> IIYPGTLWCGHGNKSSGPNELGRFKHT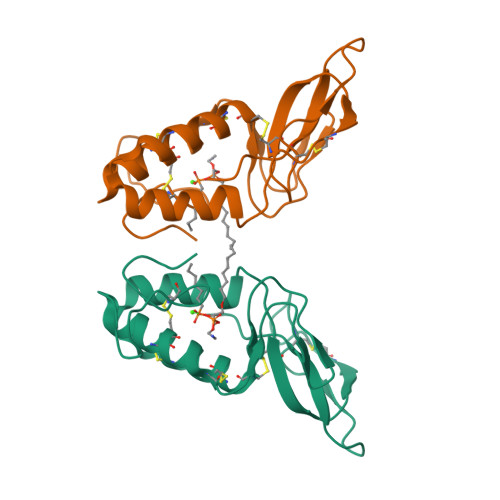DACCRTHDMCPDVMSAGESKHGLTNTASHTRLSCDCDDKFYDCLKNSADTISSYFVGKMYFNLIDTKCYKLEHPVTGCGERTEGRCLHYTVDKSKPKVYQWFDLRKY> MSTADALDDENTFKILVATDIHLGFMEKDAVRGNDTFVTLDEILRLAQENEVDFILLGGDLFHENKPSRKTLHTCLELLRKYCMGDRPVQFEILSDQSVNFGFSKFPWVNYQDGNLNISIPVFSIHGNNDDPTGADALCALDILSCAGFVNHFGRSMSVEKIDISPVLLQKGSTKIALYGLGSIPDERLYRMFVNKKVTMLRPKEDENSWFNLFVIHQNRSKHGSTNFIPEQFLDDFIDLVIWGHEHECKIAPTKNEQQLFYISQPGSSVVTSLSPGEAVKKHVGLLRIKGRKMNMHKIPLHTVRQFFMEDIVLANHPDIFNPDNPKVTQAIQSFCLEKIEEMLENAERERLGNSHQPEKPLVRLRVDYSGGFEPFSVLRFSQKFVDRVANPKDIIHFFRHREQKEKTGEEINFGKLITKPSEGTTLRVEDLVKQYFQTAEKNVQLSLLTERGMGEAVQEFVDKEEKDAIEELVKYQLEKTQRFLKERHIDALEDKIDEEVRRFRETRQKNTNEEDDEVREAMTRARALRSQSEESASAFSADDLMSIDLAEQMANDSDDSISAATNKGRGRGRGRRGGRGQNSASR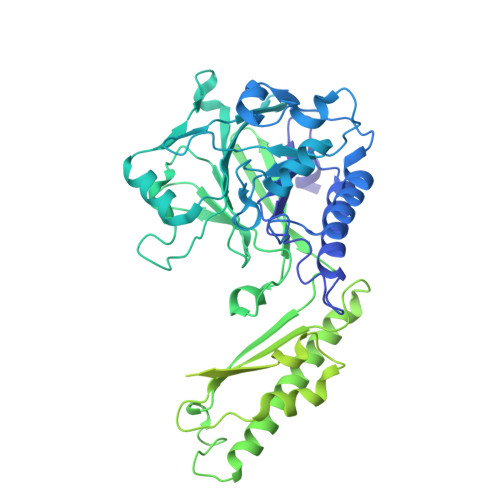GGSQRGRADTGLETSTRSRNSKTAVSASRNMSIIDAFKSTRQQPSRNVTTKNYSEVIEVDESDVEEDIFPTTSKTDQRWSSTSSSKIMSQSQVSKGVDFESSEDDDDDPFMNTSSLRRNRRSGGSLEVLFQGPDYKDDDDKGTDYKDDDDK>MGTHMYSEQGINNTINISTTSLTNATQLTVIGNNNSVYIGNNCKIVSSNIRLKGNNITLFIADDVEIMGLVCSLHSDCSLQIQAKTTMGNGEITIAEKGKISIGKDCMLAHGYEIRNTDMHPIYSLENGERINHGKDVIIGNHVWLGRNVTI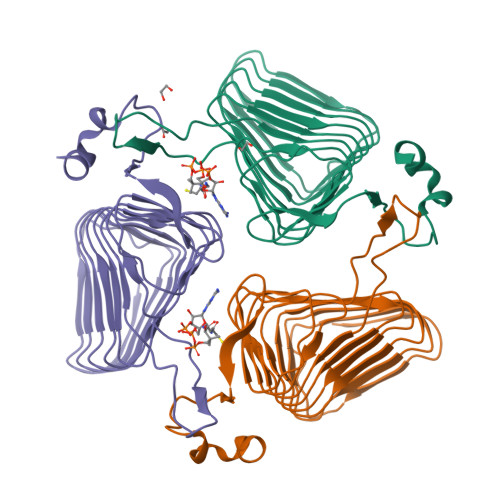LKGVCIPNNVVVGSHTVLYKSFKEPNCVIAGSPAKIVKENIVWGRKMYHSTMYDDPTLNEFYK[3x]> GIDPFTDIYDLEDLKKNLMTEGDMKIRKTDIPERYQELRAGITDYGNMSSEDQELERNWIAEKISVDKNFDANYDLTEFKEAIGNAIKFITKENLEVPFIYAYRRNYISSREKDGFLLTEDDLWDIVSLDIEFHSLVNKKDYVQRFYAELHIDDPIVTEYFKNQNTASIAELNSLQDIYDYLEFKYANEINEMFINHTGKTGKKHLKNSSYEKFKASPLYQAVSDIGISAEDVGENISSQHQIHPPVDHPSSKPVEVIESILNANSGDLQVFTSNTKLAIDTVQKYYSLELSKNTKIREKVRSDFSKYYLADVVLTAKGKKEIQKGSLYEDIKYAINRTPMHFRRDPDVFLKMVEAESLNLLSVKLHMSSQAQYIEHLFQIALETTNTSDIAIEWNNFRKLAFNQAMDKIFQDISQEVKDNLTKNCQKLVAKTVRHKFMTKLDQAPFIPNVRDPKIPKILSLTCGQGRFGADAIIAVYVNRKGDFIRDYKIVDNPFDKTNPEKFEDTLDNIIQSCQPNAIGINGPNPKTQKFYKRLQEVLHKKQIVDSRGHTIPIIYVEDEVAIRYQNSERAAQEFPNKPPLVKYCIALARYMHSPLLEYANLTSEEVRSLSIHPHQNLLSSEQLSWALETAFVDIVNLVSVEVNKATDNNYYASALKYISGFGKRKAIDFLQSLQRLNEPLLARQQLITHNILHKTIFMNSAGFLYISWNEKRQKYEDLEHDQLDSTRIHPEDYHLATKVAADALEYDPDTIAEKEEQGTMSEFIELLREDPDRRAKLESLNLESYAEELEKNTGLRK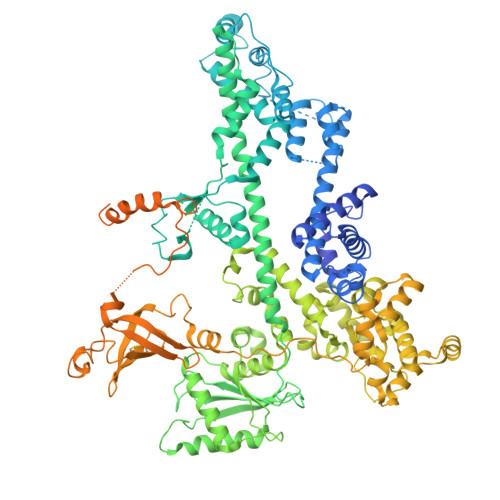LNNLNTIVLELLDGFEELRNDFHPLQGDEIFQSLTGESEKTFFKGSIIPVRVERFWHNDIICTTNSEVECVVNAQRHAGAQLRRPANEIYEIGKTYPAKVIYIDYANITAEVSLLDHDVKQQYVPISYSKDPSIWDLKQELEDAEEERKLMMAEARAKRTHRVINHPYYFPFNGRQAEDYLRSKERGEFVIRQSSRGDDHLVITWKLDKDLFQHIDIQELEKENPLALGKVLIVDNQKYNDLDQIIVEYLQNKVRLLNEMTSSEKFKSGTKKDVVKFIEDYSRVNPNKSVYYFSLNHDNPGWFYLMFKINANSKLYTWNVKLTNTGYFLVNYNYPSVIQLCNGFKTLLKSNSSKNRMNNYR>[2x]MTVNEMREWLRNWVANATGQSADAIDESTPMVELGLSSRDAVAMASDIEDLTGVTLTATVAFRHPTIESLATVIIEGEPEPEPYDEDEDWSRTRDVEDIAIVGVATRFPGDLNTPDEMWEALLEGKDCVTDLPEDRWTEFLDEPRIAERVKKARTRGGYLTDIKGFDSEFFALSKMEADNIDPQQRMALELTWEALEHARIPASSLRGESVGVYIGSSTNDYSFLAMSDPSIAHPYAITGTASSIIANRVSYFYDFRGPSVAVDTACSSSLVATH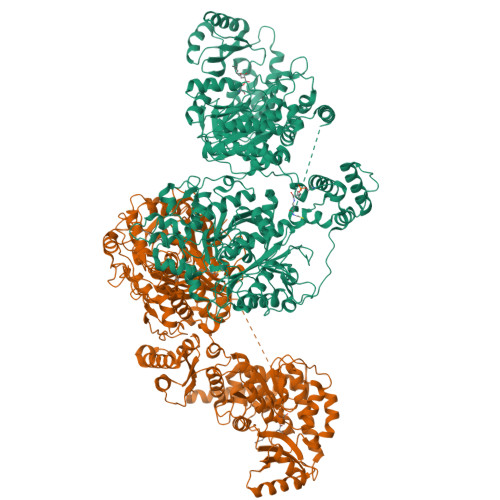QGVQALRAGEADVAIVGGVNALVTPLVTVGFDEVGGVLAPDGRIKSFSSDADGYARSEGGGMLVLKRISDARRDGDQILAVIAGSAVNHDGRSNGLLAPNPDAQAEVLRKAYKDAGINPRDVDYIEAHGTGTILGDPIEADALGRIVGKGRPADKPALLGAVKSNLGHLESAAGAASLAKMTLALANDKLPPSINYAGPNPYIDFEKERLKVNDTVSDWPRYSGKAIAGVSGFGFGGANAHVVMREVLAGDLVEPEPEPEPEAKPEKSEADAVYVGGVRMDEYGEFIDEDEPAEGGDAYPSYDEDSYELPGITEAAQRLLEQAREELEAKEAEEPTKQLVPLAVSAFLTSRKRQAAAELADWIDSPEGRASSLESIGRSLSRRNHGRSRAVVLAHDHDEAIKGLRALAEGKQHPSVLSADGPVTNGPVWVLAGFGAQHRKMGKSLYLRNEVFAEWINKVDALIQDERGYSILELILDDNVDYTDATCEYPIEVVQLVIFAIQIALGELLRHHGAKPAAVVGQSLGEAAASYFAGGLSLADATRTICSRSHLMGEGEAMLFGEYIRLMALVEYSADEIKTVFSDYPDLEVCVYAAPTQTVIGGPPDQVDAIIARAESEGKFARKFQTKGASHTQQMDPLLGELAAELQGIEPKPLTTGYFSTVHEGTFIRPGSAPIHDVDYWKKGLRHSVYFTQGIRNAVDNGHTTFLELAPNPVALMQVGLTTASAGLHDAQLIATLARKQDEVESMISAMAQLYVHGHDLDFRTLFPRRSKGLAGALDFANIPPTRFKRKEHWLPAHFTGDSSAVMPGNHVATPDGRHVWEFVPRGKTDLAALVKAAAAQVLPDAKLAAFEQRAVPADNARLVTTLTRHPGGATVQVHARVEESFTLVYDAIVARANGAGVTALPVAVGAGVAVSGDVAGEGAGASVIEDDEPDAEILQDNLTAGAGMGADFQKWDPNSGETIGQRLGTIVGAAMGYEPEDLPWEVPLIELGLDSLMAVRIKNRVEYDFDLPPIQLTAVRDANLYNVEELIRYAIEHRDEVEQIAESQKGKTAEEIAAEQSELLGGASTVAELEAKLAEAGHPLAAKDSEDSENSEDNAAGAAAAAEASAVEGLEIPPPPTDPTGPGGAPIPPPPSDPSGPAQAASATDAPAGTVNKATAAAAAAKVLTQEAVTEALGADVPPRDAAERVTFATWAIVTGKSPGGIFNELPTVSEETAKKMAERLSERAEGTITVEDVLGAKTIEGLATIVREQLEEGVVDGFVRTLRPPKEGSNAVPLFVFHPAGGSTVVYEPLMKRLPADVPVYGLERVEGSIEERAAEYVPKLLEMHKGPFVLAGWSLGGALAYACAIGLKQSGADVRFVGLIDTVLPGEPIDQSKEGMRARWDRYARFAERTFNVEIPAIPYEELEKLDDEGQVKYVLEIVKESGVQIPGGIIEHQRTSYLDNRALDTVDIKPYDGHVTLYMADRYHDDAIVFEPAYATRKPDGGWGSFVSDLEVVHIGGEHIQAIDEPYIAKVGAHMSEALNRIEAQASKEDGAK1-{4-amino-3-[6-(cyclopropyloxy)naphthalen-2-yl]-1H-pyrazolo[3,4-d]pyrimidin-1-yl}-2-methylpropan-2-ol | C22 H23 N5 O2 | 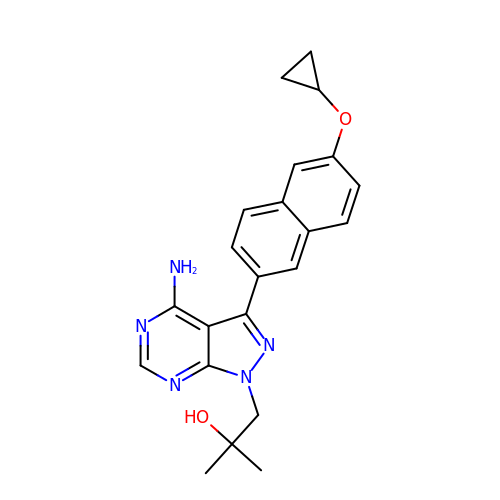NYCAEKAKFOSFFT-UHFFFAOYSA-N>TTIVSVRRNGHVVIAGDGQATLGNTVMKGNVKKVRRLYNDKVIAGFAGGTADAFTLFELFERKLEMHQGHLVKAAVELAKDWRTDRMLRKLEALLAVADETASLIITGNGDVVQPENDLIAIGSGGPYAQAAARALLENTELSAREIAEKALDIAGDICIYTNHFHTIE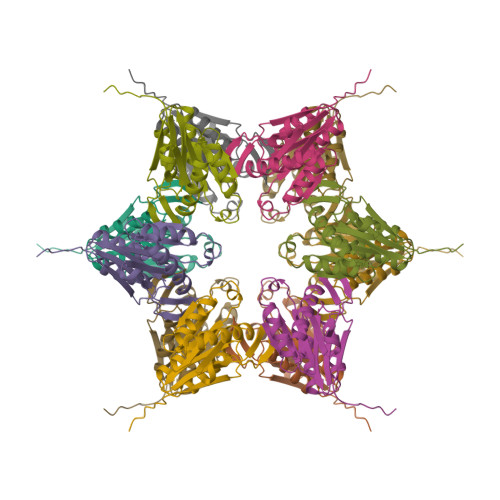ELSYKAEFHHHHHH[3x]> DNDSVVEEHGQLSISNGELVNERGEQVQLKGMSSHGLQWYGQFVNYESMKWLRDDWGINVFRAAMYTSSGGYIDDPSVKEKVKEAVEAAIDLDIYVIIDWHILSDNDPNIYKEEAKDFFDEMSELYGDYPNVIYEIANEPNGSDVTWGNQIKPYAEEVIPIIRN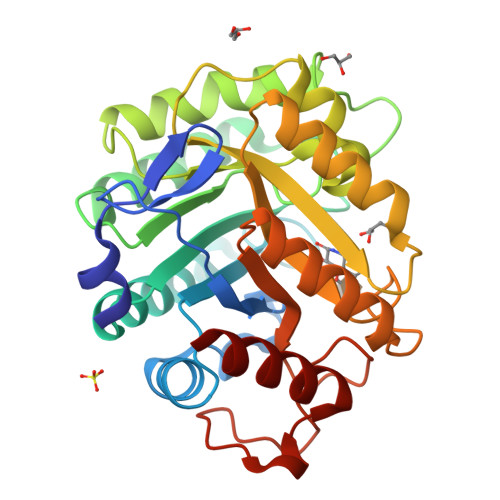NDPNNIIIVGTGTWSQDVHHAADNQLADPNVMYAFHFYAGTHGQNLRDQVDYALDQGAAIFVSEWGTSAATGDGGVFLDEAQVWIDFMDERNLSWANWSLTHKDESSAALMPGANPTGGWTEAELSPSGTFVREKIRESAS> MKYNNHDKIRDFIIIEAYMFRFKKKVKPEVDMTIKEFILLTYLFHQQENTLPFKKIVSDLCYKQSDLVQHIKVLVKHSYISKVRSKIDERNTYISISEEQREKIAERVTLFDQIIKQFNLADQSESQMIPKDSKEFLNLMMYTMYFKNIIKKHLTLSFVEFTILAIITSQNKNIVLLKDLIETIHHKYPQTVRALNNLKKQ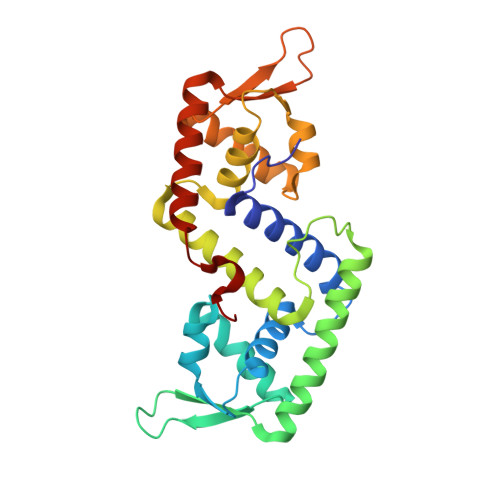GYLIKERSTEDERKILIHMDDAQQDHAEQLLAQVNQLLADKDHLHLVFE> MAHHHHHHGSRFLIRLVPEDKDRAFKVPYNHQYYLQGLIYNAIKSSNPKLATYLHEVKGPKLFTYSLFMAEKREHPKGLPYFLGYKKGFFYFSTCVPEIAEALVNGLLMNPEVRLWDERFYLHEIKVLREPKKFNGSTFVTLSPIAVTVVRKGKSYDVPPMEKEFYSIIKDDLQDKYVMAYGDKPPSEFEMEVLIAKPKRFRIKPGIYQ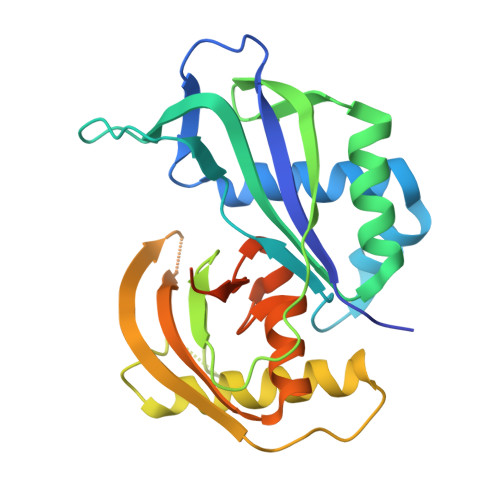TAWHLVFRAYGNDDLLKVGYEVGFGEKNSLGFGMVKVEGNKTTKEAEEQEKITFNSREELKTGV> GSSIAERSVPIAVPVPTGGDDPTKIAMLGLTFDDVLLLPAASDVLPANADTSSQLTKKIRLKVPLVSSAMDTVTEARMAIAMARAGGMGVLHRNLPVAEQAAQVETVKRSGGLLVGAAVGVGDDAWERAMALRDAGVDVLVVDTAHAHNRKVLDMVHRLKTTVGDEIEVVGGNVATRAAAAALVEAGADAVKVGVGPGSICTTRVVAGVGAPQITAILEAVAACAPHGVPVIADGGLQYSGDIAKALAAGASTAMLGSLLAGTAESPGELILVNGKQFKSYRGMGSLG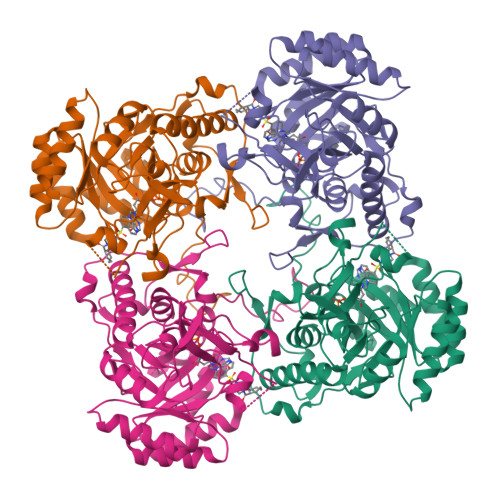AMQGRGGAKSYSKDRYFQDDALSEDKLVPEGIEGRVPFRGPLSTVIHQLVGGLRAAMGYTGSATIEELQQAQFVQITAAGLKESHPHDITMTVEAPNYYAR> MVKLRDWQEKLKDKVIEGLRNNFLVALNAPTGSGKTLFSLLVSLEVKPKVLFVVRTHNEFYPIYRDLTKIREKRNITFSFLVGKPSSCLYAEKGAESEDIPCKYCELKGSIVEVKTDDSPLSLVKKLKKDGLQDKFCPYYSLLNSLYKADVIALTYPYFFIDRYREFIDIDLREYMIVIDEAHNLDKVNELEERSLSEITIQMAIKQSKSEESRRILSKLLNQLREVVLPDEKYIKVENVPKLSKEELEILADDYEDIRKDSLKQGKVNKIHIGSILRFFSLLSIGSFIPFSYSKRLVIKNPEISYYLNLLNDNELS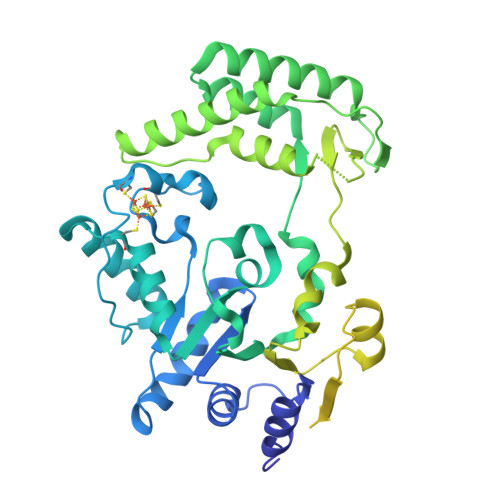IILMSGTLPPREYMEKVWGIKRNMLYLDVEREIQKRVSGSYECYIGVDVTSKYDMRSDNMWKRYADYLLKIYFQAKANVLVVFPSYEIMDRVMSRISLPKYVESEDSSVEDLYSAISANNKVLIGSVGKGKLAEGIELRNNDRSLISDVVIVGIPYPPPDDYLKILAQRVSLKMNRENEEFLFKIPALVTIKQAIGRAIRDVNDKCNVWLLDKRFESLYWKKNLKCLNANKMKL> MGYLCNDYGYEPNVDYPNASHAGLYDRSKQPYVDTAIGPKTTIQFDHVFIKSDFKTWLAHNQDEAILLIRLYELGLLLQGRSDSFLEFYNNTTYITRTDSKQPMMNKYGKLVDTTSVTCLDIFLSVVLFALNQIDSMICDFKNTPWINLSKEHKKIYELVRGIFGICYGEKDYNRFEYCPFDANSTASALNVNATLNAKKTIELITCGLIRALIAYANLVTAFSADKTALLHEILLTKVCC

Viral occlusion bodies (OBs), also called polyhedra, are stable protein crystals that encapsulate newly assembled virions within virus-infected cells. The crystalline polyhedra is formed by repeating units of the ~27.5 kDa ToNV polyhedrin protein, which is predominantly helical, containing ten helices and a short two-stranded antiparallel beta sheet. The ToNV polyhedrin structure is almost completely helical, with a 3D fold not previously observed (to the best of our knowledge). The ToNV polyhedrin achieves the first requirement by forming a dense lattice, free from continuous channels, maintained in all directions by disulfide bonds, hydrophobic and electrostatic interactions, and domain swapping.

To generate experimental phases, the wild-type ToNV polyhedrin protein was cloned into an insect cell expression vector before three hydrophobic residues (F104/L105/L137) were mutated to methionine. The native sequence contains only an N-terminal methionine. The structure was determined using single wavelength anomalous diffraction (SAD) data measured using the nano/microfocus X-ray diffraction beamline VMXm at Diamond Light Source that employs a low-background, in-vacuum cryogenic sample environment. X-ray diffraction data for both recombinant selenomethionine derivatised and native polyhedra were measured from protein crystals mounted on cryoelectron microscopy grids. SAD data were collected from selenomethionine crystals, with dimensions between 1–5 microns using a beam size of 3 by 4 (H × V) µm. Due to the small size of the crystals, small wedges of data were collected per crystal and then merged to form a final dataset using data from 55 crystals.We report studies on the reaction of cefiderocol and the related cephalosporins ceftazidime and cefepime with Pseudomonas aeruginosa PBP3, including inhibition measurements, protein observed mass spectrometry, and X-ray crystallography. PBP3 transpeptidases are proposed to be key targets for the cephalosporins and most other β-lactam antibiotics. Inhibition of PBP3 elicits transcription of genes involved in the SOS response, ultimately leading to cell cycle arrest. Consequently, PBP3 is one of the most validated and clinically important antibacterial targets.

The cephalosporin cefiderocol (Fetroja©), which was developed by Shionogi, is a pioneering example of a ‘Trojan horse’ class antibiotic: its C3′ linked catechol group acts as a siderophore enabling it to efficiently enter Gram-negative cells via the iron/siderophore transport system. The three cephalosporins form analogous 3-exomethylene products with P. aeruginosa PBP3 following elimination of the C3′ side chain. pIC50 and kinact/Ki measurements with isolated PBP3 imply ceftazidime and cefiderocol react less efficiently than cefepime and, in particular, meropenem with P. aeruginosa PBP3. The C7 oxime linked carboxylic acids of cefiderocol/ceftazidime bind identically, directly interacting with the guanidino group of Arg440, being positioned to form two salt bridges (∼2.6–3.4 Å). The C7 aminothiazole moiety appears to form identical interactions in both the cefepime and cefiderocol/ceftazidime structures. The aminothiazole amine NH2 forms hydrogen bonds with both the side chain carbonyl oxygen of Glu242 (∼3.1–3.6 Å) and the backbone carbonyl oxygen of Arg440 (∼2.8–2.9 Å). With the cephalosporin complex structures, the C7 amide oxygen is positioned to interact via a hydrogen bond with the side chain amide NH2 of Asn302 (∼2.8–3.0 Å). With cefiderocol, a small amount of cefiderocol modified PBP3 was observed, however, most of the observed complex was meropenem modified PBP3. The kinact/Ki of cefepime was slightly less than that of meropenem (9600 and 11 000 M−1 s−1, respectively), whilst the kinact/Ki values of cefiderocol and ceftazidime were similar and substantially lower (3000 and 3400 M−1 s−1, respectively). Given that the siderophore group of cefiderocol is lost on reaction with PBP3, it is also of interest to explore whether this affects resistance, including by using analogues of cefiderocol where such loss cannot occur.

> GGSVRHIAIPAHRGLITDRNGEPLAVSTPVTTLWANPKELMTAKERWPQLAAALGQDTKLFADRIEQNAEREFIYLVRGLTPEQGEGVIALKVPGVYSIEEFRRFYPAGEVVAHAVGFTDVDDRGREGIELAFDEWLAGVPGKRQVLKDRRGRVIKDVQVTKNAKPGKTLALSIDLRLQYLAHRELRNALLENGAKAGSLVIMDVKTGEILAMTNQPTYNPNNRRNLQPAAMRNRAMIDVFEPGSTVKPFSMSAALASGRWKPSDIVDVYPGTLQIGRYTIRDVSRNSRQLDLTGILIKSSNVGISKIAFDIGAESIYSVMQQVGLGQDTGLGFPGERVGNLPNHRKWPKAETATLAYGYGLSVTAIQLAHAYAALANDGKSVPLSMTRVDRVPDGVQVISPEVASTVQGMLQQVVEAQGGVFRAQVPGYHAAGKSGTARKVSVGTKGYRENAYRSLFAGFAPATDPRIAMVVVIDEPSKAGYFGGLVSAPVFSKVMAGALRLMNVPPDNLPTEFEA>MGSDKIHHHHHHLPLFKFAIDVQYRSNVRDPRGETIERVLREEKGLPVKKLRLGKSIHLEVEAENKEKAYEIVKKACEELLVNP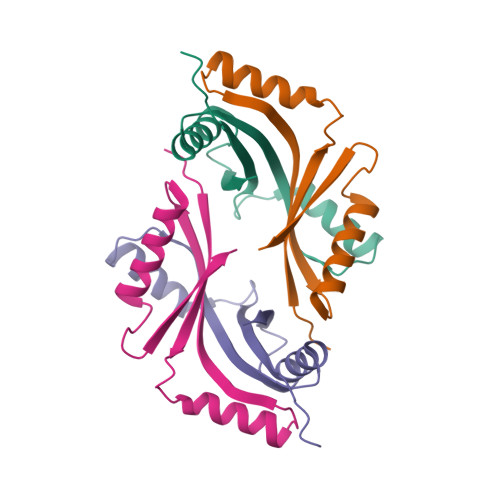VVEEYEVREL[4x]> MTDHARGTLPEIRRGRIYRDVYHKRVDEEPVDRTADLERARLGDDGLDFQDDAAQARAFAQGVFLLEIPEWLDLSAGDRFARQFFQGTGVEPYGKYRDLSSEHFGDELLGYHSRVDQLEQFLLERRFWGEVYPSEIATLGEHLTLLSHRVLRSVLASAGI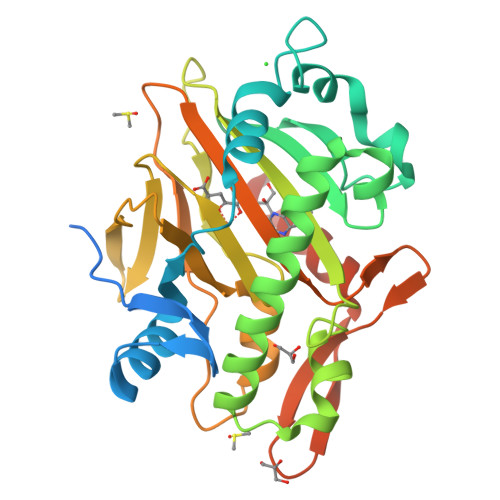PEEDWHRASGGCSETNGSYHLTFNHYRSAHQDIGLSSHKDDGFITVLRTTAQGLEVNRDDVWEKVPVDPACFVVNFGLSMEILTSACVTPLSAIMHRVSHQNFDRSSFGHFSSSRCLPGADDGIYRYLPSAGLERVCGSRELIEENDHEIYMGTEGQGLEHHHHHHHH> MQVSSSFRSFLKLDILHSYF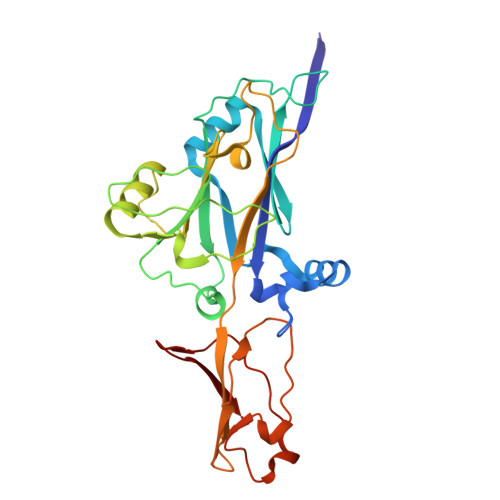LNDGEKDFSSMNEEESKTQLKSYNWKDFLEIYPSQKTSHMMRGNKIFFKSFNDSIILAIKVESGTENQPFNELYEDESMTFLLSLKDQYFGNYTDLDLADQLLYFSNKTPVLPEAFTFKPIDRINQSGTVGEEYLYEGENKKHLLEEAHLNPGGGVLGIIQIYMKGDTPVLSLINNDGTLKNSLPHFKIHFSNRKSTWKYINLKDDFETETKKDYPLTKFGFILLDKKSDFISPPAHFEKYVFPNPDARRIKITPTKNYSEIFI>[3x]MRKLLPILIGLSLSGFSSLSQAENLMQVYQQARLSNPELRKSAADRDAAFEKINEARSPLLPQLGLGADYTYSNGYRDANGINSNATSASLQLTQSIFDMSKWRALTLQEKAAGIQDVTYQTDQQTLILNTATAYFNVLNAIDVLSYTQAQKEAIYRQLDQTTQRFNVGLVAITDVQNARAQYDTVLANEL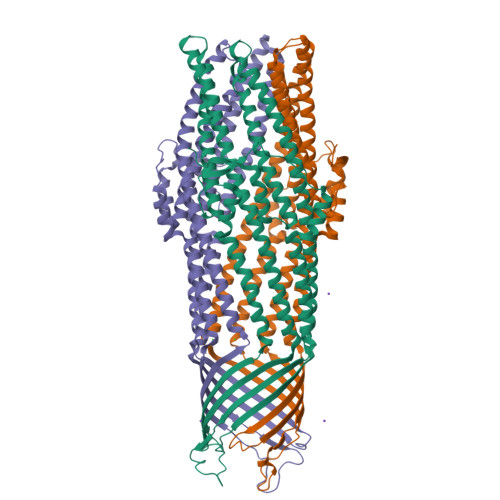TARNNLDNAVEQLRQITGNYYPELAALNVENFKTDKPQPVNALLKEAEKRNLSLLQARLSQDLAREQIRQAQDGHLPTLDLTASTGISDTSYSGSKTRGAAGTQYDDSNMGQNKVGLSFSLPIYQGGMVNSQVKQAQYNFVGASEQLESAHRSVVQTVRSSFNNINASISSINAYKQAVVSAQSSLDAMEAGFSVGTETIVDVLDATTTLYNAKQELANARYNYLINQLNIKSALGTLNEQDLLALNNALSKPVSTNPELEHHHHHHHH>QQPGTSTPEVHPKLTTYKCTKSGGCVAQDTSVVLDWNYRWMHDKNFNSCTVNGGVNTTLCPDEATCGANCFIEGVDYAASGVTVSGSSLTMNQYMPSSSGGYSSVSPRLYLLGSDGDYELLQLNGQELSFDVDLSTLPCGENGALYLSEMAANGGANQYNTAGANYGSGYCDAQCPVQTWKNGTLNTNHSGYCCNEMDILEANSRANAFTPHSCTATACDASGCGFNPYANGFQRYWGPGFTLDTSKVFTIITQFNTDNGLPSGNLVSITRKYRQNGVDVPSAQSGGDTISSCPSASAYGGLTTMGKALANGMVLVFSIWNDNGGNM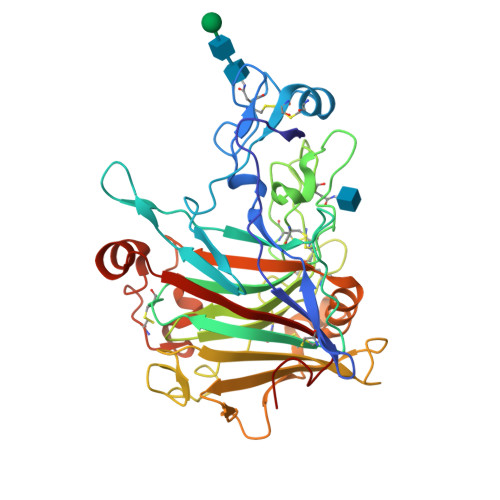NWLDSGNAGPCSSTEGNPSTIVANNPGTHVIFSNIRWGDIGSTTGG[2x]1-HEXADECANOSULFONIC 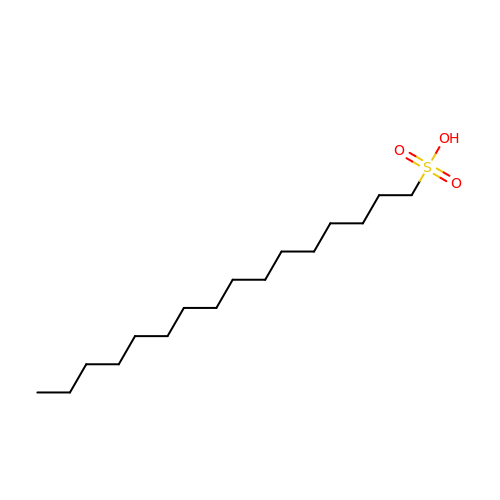ACID | C16 H34 O3 S | SSILHZFTFWOUJR-UHFFFAOYSA-N>[7x]VYTSTETS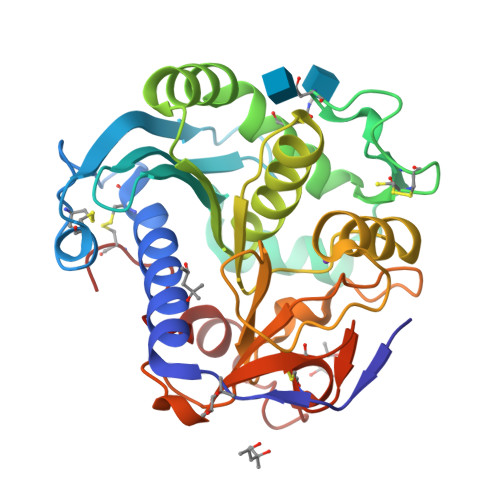HIDQESYNFFEKYARLANIGYCVGPGTKIFKPFNCGLQCAHFPNVELIEEFHDPRLIFDVSGYLAVDHASKQIYLVIRGTHSLEDVITDIRIMQAPLTNFDLAANISSTATCDDCLVHNGFIQSYNNTYNQIGPKLDSVIEQYPDYQIAVTGHSLGGAAALLFGINLKVNGHDPLVVTLGQPIVGNAGFANWVDKLFFGQENPDVSKVSKDRKLYRITHRGDIVPQVPFWDGYQHCSGEVFIDWPLIHPPLSNVVMCQGQSNKQCSAGNTLLQQVNVIGNHLQYFVTEGVCGI>GSHEEENDVVKGNFDISKISGDWY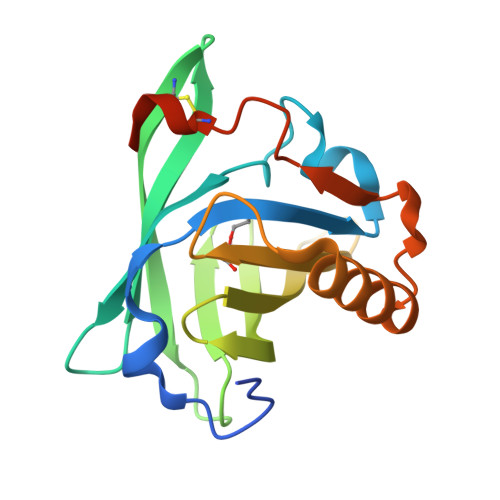SILLASDIKEKIEENGSMRVFVKDIEVLSNSSLIFTMHTKVNGKCTKISLICNKTEKDGEYDVVHDGYNLFRIIETAYEDYIIFHLNNVNQEQEFQLMELYGRKPDVSPKVKEKFVRYCQGMEIPKENILDLTQVDRCLQARQSEAAQVSSAE[4x]> MSDKRKIQHEGIIALINYSTLCAQKCDVLKGHDDKIT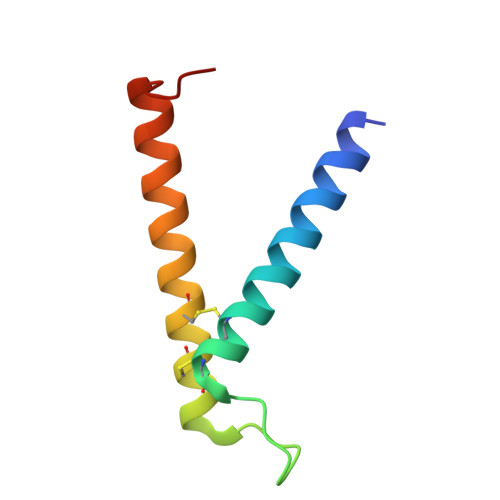DTEEQCLRVCAEKIRQTFEFTNDIYLKNPNLTKPN>MSTVVQQVPAELQAALTLINNDPRMRTNNAWALSADKRWSLKFTAELSVPCSSFMPDNSVWHLVLWQEETLIRIEVYPDKSEGISATFQHQNYNFSDASTREWTSGNPALENTPTVFGRNLWGLEPEALLDRISWRLSRLLLWIDAAAQEKLATTGDAVELPAFPDQSPFTVIGFSEQIDDLPFWASKTGEWGFASSTGLPGAHGTLFLREFLDNKGKLIRTTKWSPFMRKGARTTNAVWSVLPTLPVLAPWQAPRTWQELSHCFAQCGLSLPDLFSDIGRSVRALRKQRAPGLLLLGFPLENKIGDEPARIHWLALRLAGLSNTMTKRPGFRPTERNRRTWDREQPLSQEPIRWVRTQNWAADQLRTRGEAANDIRSKKVLIIGAGSLGSMIAENLMRIGVVSQGILDADLLQTGNLSRHALTMTSVGHNKAAALVEHLNRILPDASARSFSCAFPPESEVAKNSLRQYDVIIDCTGDDGVLKSLAAFDWKSEKIFISLAMTWRAEGLFAFAASETSFPVTDASSRFNASASPEIDMDEARIEGIGAWHPVFPARADDVQLWAAVGTKFICRVVSAPGRIYEYFKQMPDGTVEKEPHEY[2x]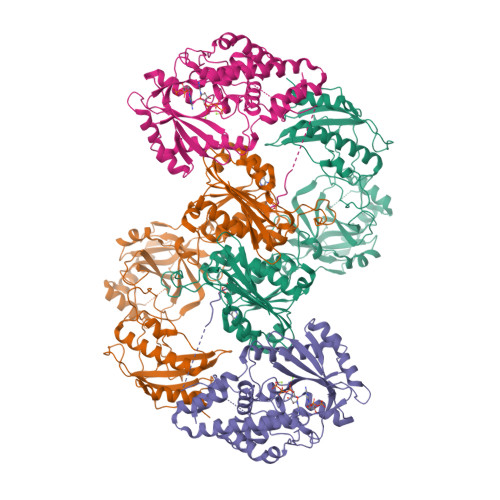;>[2x]MKSSHHHHHHENLYFQSNAELQPQFNEFLANIRPTDTQKEDWKSGARTLRERLKNFEPLKEIVVSTFLQGSIRRSTAIRPLGDKRPDVDIVVVTNLDHTRMSPTDAMDLFIPFLEKYYPGKWETQGRSFGITLSYVELDLVITAIPESGAEKSHLEQLYKSESVLTVNSLEEQTDWRLNKSWTPNTGWLSESNSAQVEDAPASEWKAHPLVLPDREKNEWGRTHPLAQIRWTAEKNRLCNGHYINLVRAVKWWRQQNSEDLPKYPKGYPLEHLIGNALDNGTTSMAQGLVQLMDTFLSRWAAIYNQKSKPWLSDHGVAEHDVMARLTAEDFCSFYEGIASAAEIARNALASEEPQESAQLWRQLFGSKFPLPGPQGGDRNGGFTTPSKPAEPQKTGRFA>GSETLVRPKPELLKLLKSVGAQKDTYTMKEVLFYLGQYIMTKRLYDEKQQHIVYCSNDLL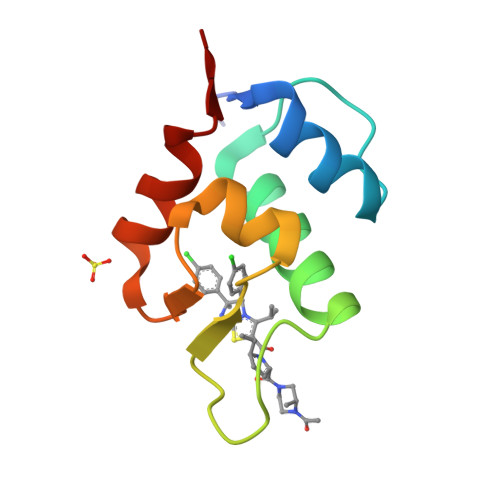GDLFGVPSFSVKEHRKIYTMIYRNLVV[2x]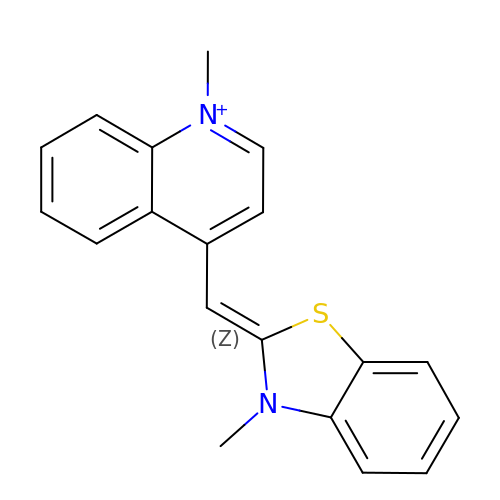1-methyl-4-[(Z)-(3-methyl-1,3-benzothiazol-2(3H)-ylidene)methyl]quinolin-1-ium | C19 H17 N2 S | XRXJDLHDDHBJOJ-UHFFFAOYSA-N>GPHMQPDPYQILGPTSSRLANPGSGQIQLWQFLLELLSDSANASCITWEGTNGEFKMTDPDEVARRWGERKSKPNMNYDKLSRALRYYYDKNIMTKVHGKRYAYKFDFHGIAQALQPHPTESSMYKYPSDISYMPS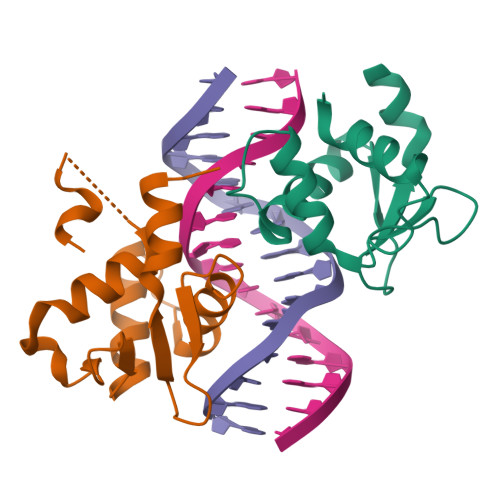YHAHQQKVN[2x]>[6x]MGSDK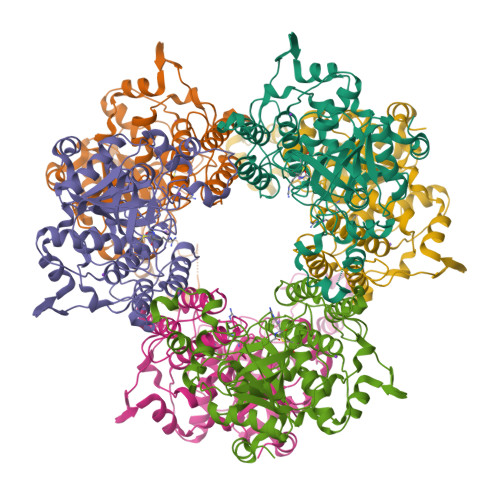IHHHHHHENLYFQQDTEKKVSEEGFVFTTVKENPITSVKNQNRAGTCWCYSSYSFLESELLRMGKGEYDLSEMFTVYNTYLDRADAAVRTHGDVSFSQGGSFYDALYGMETFGLVPEEEMRPGMMYADTLSNHTELSALTDAMVAAIAKGKLRKLQSDENNAMLWKKAVAAVHQIYLGVPPEKFTYKGKEYTPKSFFESTGLKASDYVSLTSYTHHPFYTQFPLEIQDNWRHGMSYNLPLDEFMEVFDNAINTGYTIAWGSDVSESGFTRDGVAVMPDDEKVQELSGSDMAHWLKLKPEEKKLNTKPQPQKWCTQAERQLAYDNYETTDDHGMQIYGIAKDQEGNEYYMVKNSWGTNSKYNGIWYASKAFVRYKTMNIVVHKDALPKAIKAKLGIK> MISTPLSKEFEWPAKPVSLELQHQVEQFYYREAQLLDHHAFQAWFA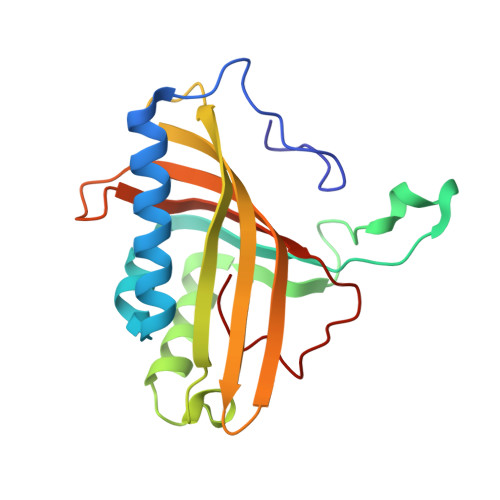LLAEDIHYWMPIRTVRTAREQGLEYVPAGANAHFDDTHATMYGRIRQKTSDLNWAEDPPSRTRHLVSNVIVREMDTPGTLEVASAFLLYRSRLERQVDVFAGERRDVLRIADNPLGFQIAKRTIILDQSTVLANNLSVFF> MKELFEVIFEGVNTSRLFFLLKEIESKSDRIFDFNFSEDFFSSNVNVFSELLIDSFLGFNGDLYFGVSMEGFSVKDGLKLPVVLLRVLKYEGGVDVGLCFYMNDFNSAGKVMLEFQKYMNGISADFGFENFYGGLEPASDQETRFFTNNRLGP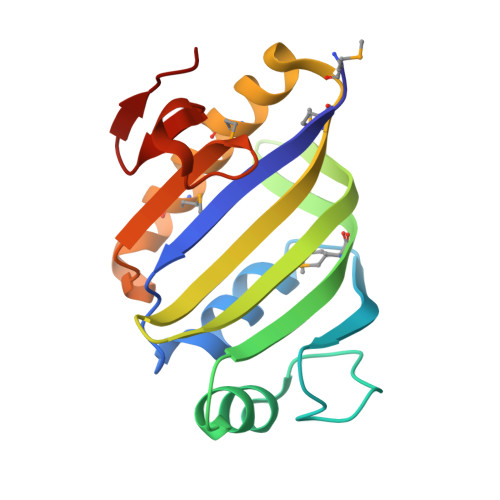LL>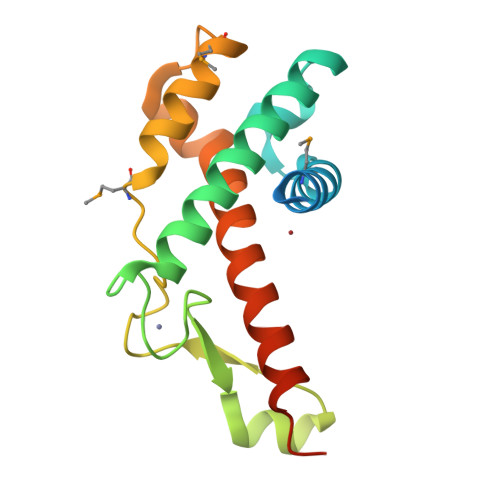MGMAQSQAGFGMAAFCGKHELSQNDKQKAINYLMQFAHKVSGKYRGVAKLEGNTKAKVLQVLATFAYADYCRSAATPGARCRDCHGTGRAVDIAKTELWGRVVEKECGRCKGVGYSRMPASAAYRAVTMLIPNLTQPTWSRTVKPLYDALVVQCHKEESIADNILNAVTRLEHHHHHH[2x]> ESTPIQQLLEHFLRQLQRKDPHGFFAFPVTDAIAPGYSMIIKHPMDFGTMKDKI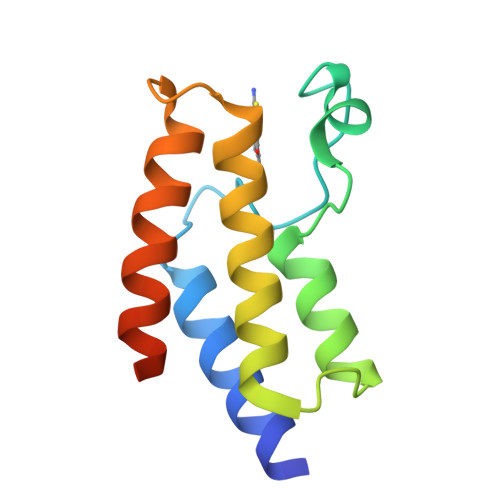VANEYKSVTEFKADFKLMCDNAMTYNRPDTVYYKLAKKILHAGFKMMSKLEHHHHHH>[2x]MAHH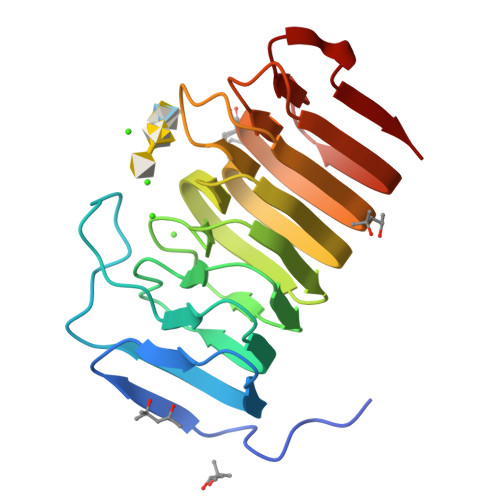HHHHVGTNTGGVLVITDTIIVKSGQTYDGKGIKIIAQGMGDGSQSENQKPIFKLEKGANLKNVIIGAPGCDGIHCYGDNVVENVVWEDVGEDALTVKSEGVVEVIGGSAKEAADAVFALNAPCTFKVKNFTATNIGKLVRQNGNTTFKVVIYLEDVTLNNVKSCVAKSDSPVSELWYHNLNVNNCKTLFEFPSQSQIHQY>[2x]GPHMAR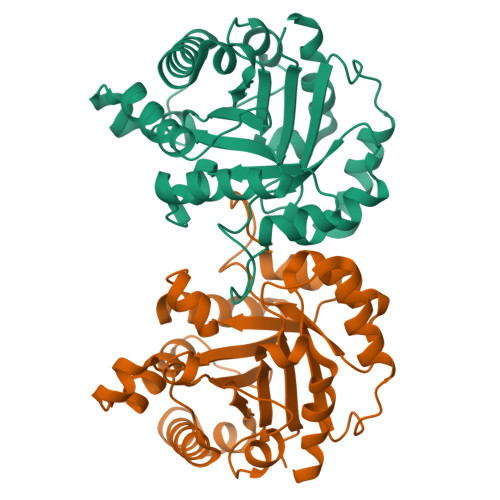KFFVGGNWKCNGTAEEVKKIVNTLNEAQVPSQDVVEVVVSPPYVFLPLVKSTLRSDFFVAAQNCWVKKGGAFTGEVSAEMLVNLDIPWVILGHSERRAILNESSEFVGDKVAYALAQGLKVIACVGETLEEREAGSTMDVVAAQTKAIADRVTNWSNVVIAYEPVWAIGTGKVASPAQAQEVHDELRKWLAKNVSADVAATTRIIYGGSVNGGNCKELGGQADVDGFLVGGASLKPEFIDIIKAAEVKKSA>MTTPSMEDYIEQIYMLIEEKGYARVSDIAEALAVHPSSVTKMVQKLDKDEYLIYEKYRGLVLTSKGKKIGKRLVYRHELLEQFLRIIGVDEEKIYNDVEGIEHHLSWNSIDRIGDLVQYFEEDDARKKD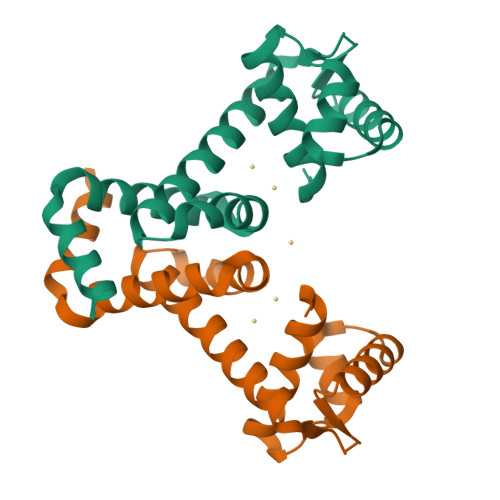LKSIQKKTEHHNQ[2x]> MKRIVVPHRWSEMNRVEHPPLMMKQLFQGVCGGLRWLETKSLAQYLAVRAIEEGYPSTPG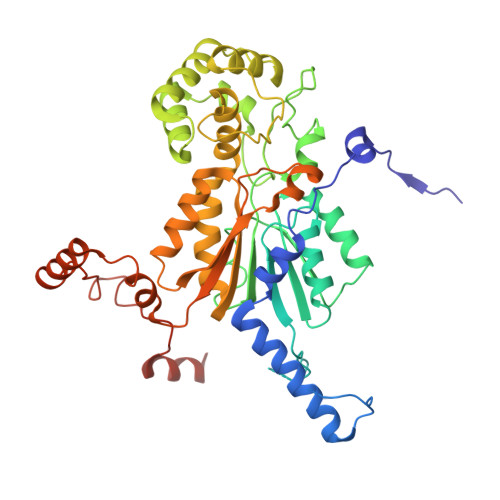VRKALHVKRAPLQKRRVVQRSTKSATAACSLPTTAAPAQLPLTSSGDALTVTGGLSLQVTKQKRLVSYDVLDCTLGSGYHAGAVLENGGPYTRVVALDCDHDAMHAARDLVEEFGGDRFRFYCCKMSEAKAMFGERSFDAIMIDGGVSDTQLEDPERGFLLDDEGGHRLDMRFGPQMGVGALEYLNTVSQHTLVSSLLAYGLLEYGQAMKMSRAITRRKPFVDSREVLTCIEQAGDELPEGGWRSQGSRRKSPMSWKFLTSLRCIINNEMYELRQGIENALLMLRDDGRLVVFSRLPWEERLVRGTVDDHPHALLSYVEDISIDDVQIYGFTRHAKMWVITRAASSAYALKNTTTLTEEKFRESSVRWLTGMYAGQTHGFPANNFTFENFERKEWVTLRRNGKPPPVDVGLDDK> MLARRKKVYPYPMEPTI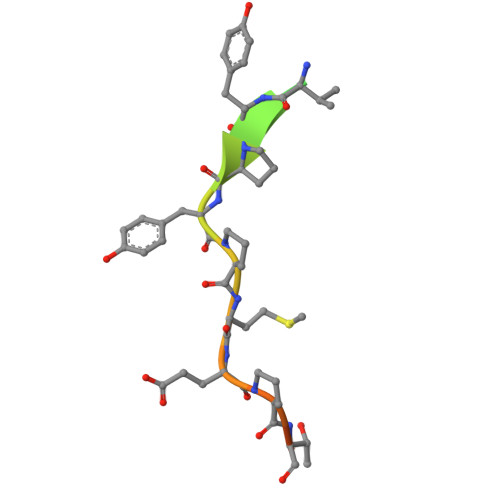AEG>MRNEMHLQFSARSENESFARVTVAAFVAQLDPTMDELTEIKTVVSEAVTNAIIHGYNNDPNGIVSISVIIEDGVVHLTVRDEGVGIPDIEEARQPLFTTKPELERSGMGFTIMENFMDEVIVESEVNKGTTVYLKKHIVKSKRYLEGSSF[2x];> GSHMQGQSPIKDQEMKELIRRSQEGDQEARDEIIEKNMRLVWSVVQRFLNRGYEADDLFQIGCIGLLKSVDKFDLSYDVKFSTYAVPMIIGEIQRFLRDDGTVKVSRSLKEMGNKIRKAKDELSKTRGR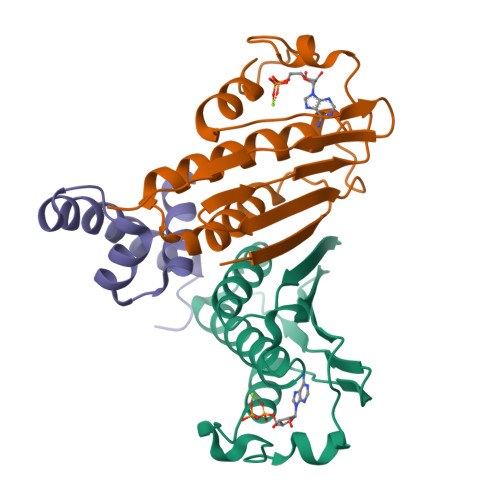APTVTEIADHLGISPEDVVLAQEAVRLPTSIHETVYENDGDPITLLDQIADADEASWFDKIALKKAIEELDERERLIVYLRYYKDQTQSEVASRLGISQVQMSRLEKKILQHIK> ASVKAVGRVCYSALPSQ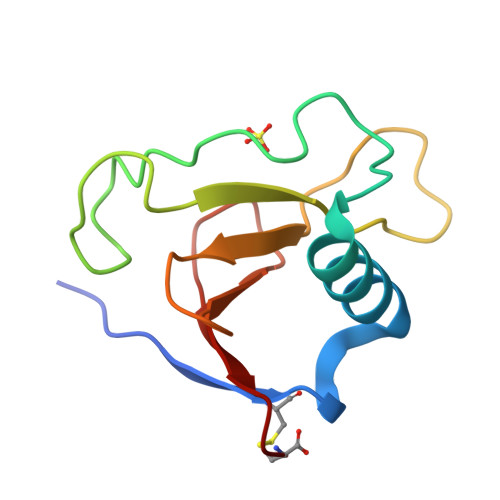AHDTLDLIDEGGPFPYSQDGVVFQNREGLLPAHSTGYYHEYTVITPGSPTRGARRIITGQQWQEDYYTADHYASFRRVDFAC>MSASIPDIKLSSGHLMPSIGFGCWKLANATAGEQVYQAIKAGYRLFDGAEDYGNEKEVGDGVKRAIDEGLVKREEIFLTSKLWNNYHDPKNVETALNKTLADLKVDYVDLFLIHFPIAFKFVPIEEKYPPGFYCGDGNNFVYEDVPILETWKALEKLVAAGKIKSIGVSNFPGALLLDLLRGATIKPAVLQVEHHPYLQQPKLIEFAQKAGVTITAYSSFGPQSFVEMNQGRALNTPTLFAHDTIKAIAAKYNKTPAEVLLRWAAQRGIAVIPKSNLPERLVQNRSFNTFDLTK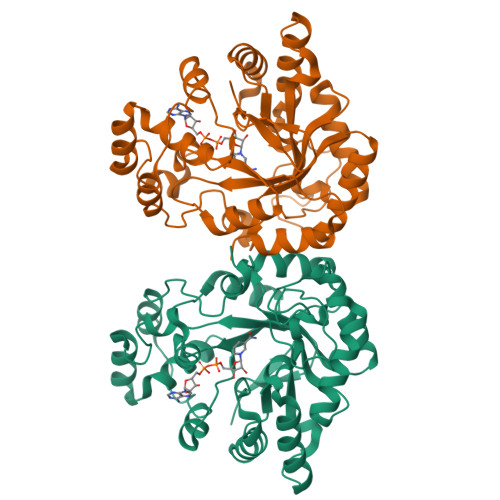EDFEEIAKLDIGLRFNDPWDWDNIPIFV[4x]> ASMKNCVIVSAVRTAIGSFNGSLASTSAIDLGATVIKAAIERAKIDSQ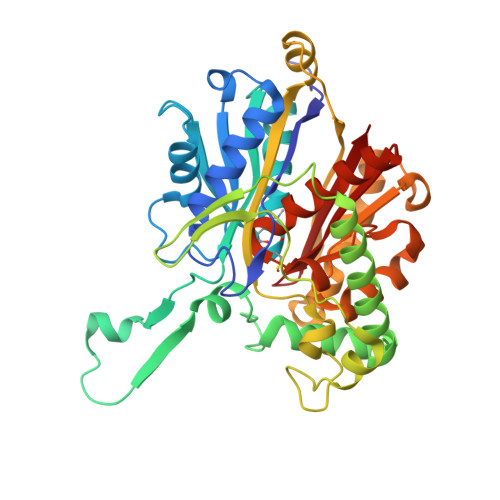HVDEVIMGNVLQAGLGQNPARQALLKSGLAETVCGFTVNKVCGSGLKSVALAAQAIQAGQAQSIVAGGMENMSLAPYLLDAKARSGYRLGDGQVYDVILRDGLMCATHGYHMGITAENVAKEYGITREMQDELALHSQRKAAAAIESGAFTAEIVPVNVVTRKKTFVFSQDEFPKANSTAEALGALRPAFDKAGTVTAGNASGINDGAAALVIMEESAALAAGLTPLARIKSYASGGVPPALMGMGPVPATQKALQLAGLQLADIDLIEANEAFAAQFLAVGKNLGFDSEKVNVNGGAIALGHPIGASGARILVTLLHAMQARDKTLGLATLCIGGGQGIAMVIER> QDNSRYTHFLTQHYDAKPQGRDDRYCEAIMRRRGLAAPCKDINTFI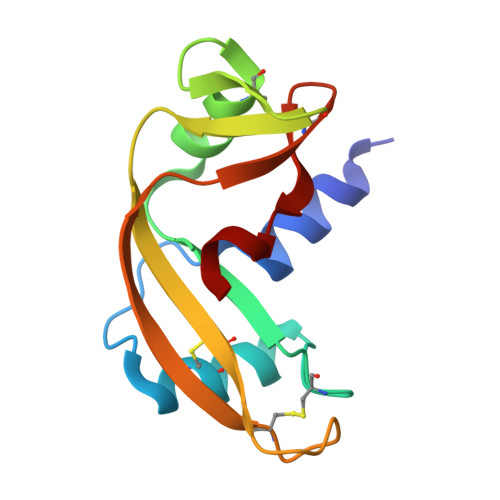HGNKRSIKAICENKNGNPHRENLRISKSSFQVTTCKLHGGSPWPPCQYRATAGFRNVVVACENGLPVHLDQSIFR>MESKRNKPGKATGKGKPVGDKWLDDAGKDSGAPIPDRIADKLRDKEFKNFDDFRKKFWKEVAKDPDLAKQFSKANQRNIKDGNAPFARESDQVGGRTTYELHHDKPISQDGGVYDMNNIRVTTPKRAIDIHRGK[2x];>[2x]MELKHSISDYTEAEFLEFVKDIFRLSRPQDNDLQIKLVLEFKRLTEHP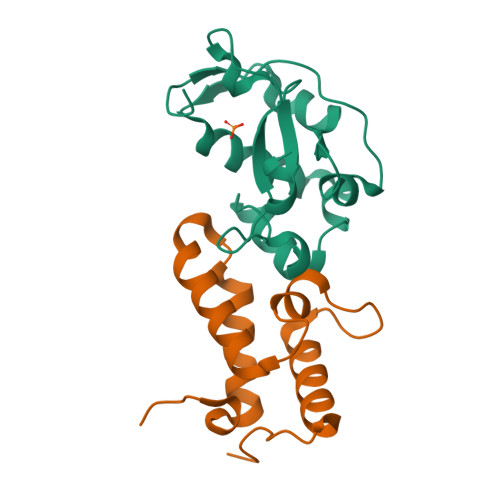DGSDLIYYPRSDREDSPEGIVKEIKEWRAANGKSGFKQGLEHHHHHH> MKDVSKNQEENISDTALTNELIHLLGHSRHDWMNKLQLIKGNLSLQKYDRVFEMIEEMVIDAKHESKLSNLKTPHLAFDFLTFNWKTHYMTLEYEVLGEIKDLSAYDQKLAKLMRKLFHLFDQAVSRESE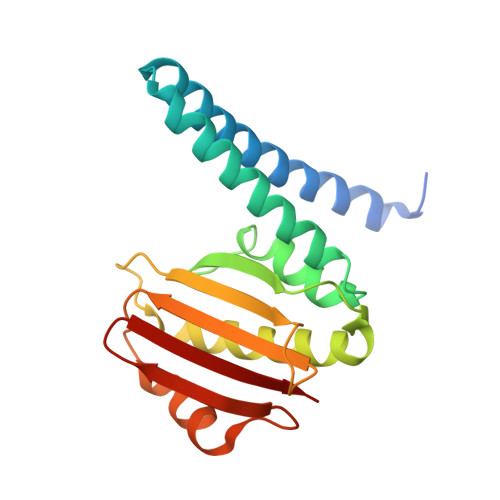NHLTVSLQTDHPDRQLILYLDFHGAFADPSAFDDIRQNGYEDVDIMRFEITSHECLIEIGLD>MNLPTAQEVQGLMARYIELVDVGDIEAIVQMYADDATVENPFGQPPIHGREQIAAFYRQGLGGGKVRACLTGPVRASHNGCGAMPFRVEMVWNGQPCALDVIDVMRFDEHGRIQTMQAYWSEVNLSVREPQ[4x]

We have systematically dissected the potential contribution to catalysis from electrostatic complementarity in ketosteroid isomerase. We first describe KSI, an enzyme suggested to provide electrostatic complementarity to the transition state via oxyanion hole hydrogen bonds. Phenolates, analogs of the transition state and reaction intermediate, bind and accept two hydrogen bonds in an active site oxyanion hole.

Further characterization of KSI via X-ray crystallography, NMR, and isothermal titration calorimetry (ITC) was more readily carried out with one or the other enzyme: pKSI for obtaining a high-resolution crystal structure and for calorimetry and tKSI for NMR spectroscopy. (A) Electron density map (1.5 σ) shows that phenolate is bound at the oxyanion hole, receiving short hydrogen bonds from Tyr16 and Asp103. Results with several spectroscopic techniques confirmed that the anionic phenolate form of the ligand, with a negatively charged oxygen, was bound rather than the unionized phenol form. (B) For phenolate, the average angles are 15° and 47°. The ability of KSI to bind phenolate ions in a mode analogous to its reaction intermediate and transition states provided an exceptional opportunity to isolate the electrostatic behavior of the KSI oxyanion hole and thereby evaluate the energetic contribution from electrostatic transition state complementarity. a, observed with enzymes from two different sources and by two independent binding assays, suggests that electrostatic complementarity in the oxyanion hole provides at most a modest catalytic contribution of ˜300-fold. The results herein indicate that hydrogen bonding in the active site of KSI provides little electrostatic advantage compared with water. In summary, electrostatic and geometrical complementarity may each play modest roles in catalysis by KSI, and there may be additional contributions from better accommodation of the steroid ring geometry in the transition state than in the ground state.4,4'-{cyclohexa-2,5-diene-1,4-diylidenebis[(E)methylylidene(E)diazene-2,1-diyl]}bis[N-(2-chlorophenyl)-4-oxobutanamide] | C28 H24 Cl2 N6 O4 | 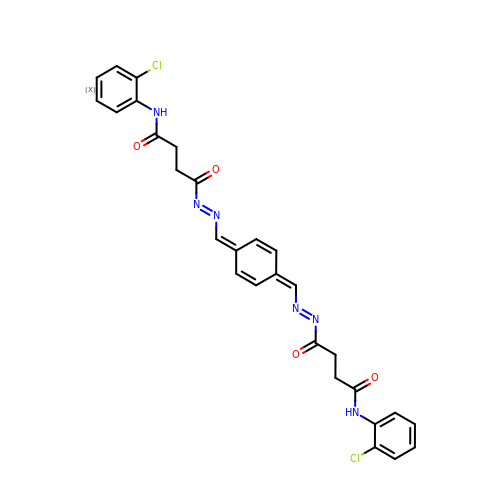HTJQQXMFDMUXSX-MDQGHDFKSA-N> MAARDFEYNNQDVNQLNGAFISLVEDEKIGFWVGVGG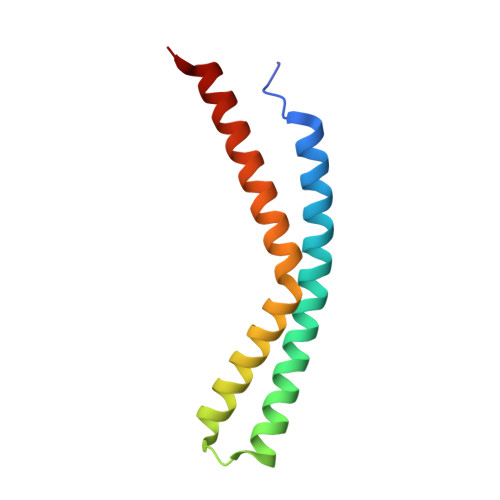FAYSQFIMRKFVKSTNIFASVTSLFAGAALANLYTHQSRASYARVAARANRNASLALNKLMEY>[4x]MSKVYVVAAKRSAIGSFLGTLSPLKPGDLGAQIVKNILEETKVDPANIDEVIVGNVLSAGQAQGVGRQVAIRAGIPYEVPAYSVNIICGSGMK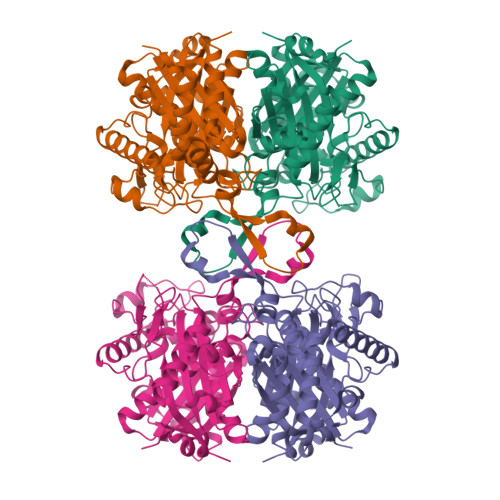SVITAFSNIKAGEADLVIAGGTESMSGAGFILPGAIRGGHKMADLTMKDHMILDALTDAYHNIHMGITAENIAERYGITREEQDAFALDSQLKAIAAVDSGRFKDEIAPVVIPNKKGDIIFDTDEYPNRKTDAEKLAKLKPAFKKDGSVTAGNASGLNDGASFLMLASEEAVKKYNLKPLVEIVATGTGGVDPLVMGMGPVPAIRKAFNKTDLKLKDMELIELNEAFAAQSLGVIKELCKEHGVTPEWIKERTNVNGGAIALGHPVGASGNRITVTLIYEMKKRGVEYGLASLCIGGGMGTALILKNVK> MGSSHHHHHHSSPISPIETVPVKLKPGMDGPKVKQWPLTEEKIKALVEICTEMEKEGKISKIGPENPYNTPVFAIKKKDSTKWRKLVDFRELNKRTQDFWEVQLGIPHPAGLKKKKSVTVLDVGDAYFSVPLDEDFRKYTAFTIPSINNETPGIRYQYNVLPQGWKGSPAIFQSSMTKILEPFRKQNPDIVIYQYVDDLYVGSDLEIGQHRTKIEELRQHLLRWGLTTPDKKHQKEPPFLWMGYELHPDKWTVQPIVLPEKDSWTVNDICKLVGKLNWASQIYPGIKVRQLSKLLRGTKALTEVIPLTEEAELELAENREILKEPVHGVYYDPSKDLIAEIQKQ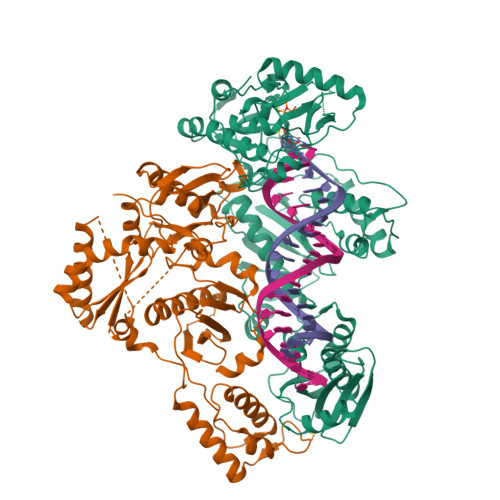GQGQWTYQIYQEPFKNLKTGKYARMRGAHTNDVKQLTEAVQKITTESIVIWGKTPKFKLPIQKETWETWWTEYWQATWIPEWEFVNTPPLVKLWYQLEKEPIVGAETFYVDGAANRETKLGKAGYVTNRGRQKVVTLTDTTNQKTELQAIYLALQDSGLEVNIVTDSQYALGIIQAQPDQSESELVNQIIEQLIKKEKVYLAWVPAHKGIGGNEQVDKLVSAGIRKVL;> PISPIETVPVKLKPGMDGPKVKQWPLTEEKIKALVEICTEMEKEGKISKIGPENPYNTPVFAIKKKDSTKWRKLVDFRELNKRTQDFWEVQLGIPHPAGLKKKKSVTVLDVGDAYFSVPLDEDFRKYTAFTIPSINNETPGIRYQYNVLPQGWKGSPAIFQSSMTKILEPFRKQNPDIVIYQYVDDLYVGSDLEIGQHRTKIEELRQHLLRWGLTTPDKKHQKEPPFLWMGYELHPDKWTVQPIVLPEKDSWTVNDIQKLVGKLNWASQIYPGIKVRQLSKLLRGTKALTEVIPLTEEAELELAENREILKEPVHGVYYDPSKDLIAEIQKQGQGQWTYQIYQEPFKNLKTGKYARMRGAHTNDVKQLTEAVQKITTESIVIWGKTPKFKLPIQKETWETWWTEYWQATWIPEWEFVNTPPLVKLWYQLEKEPIVGAETF Despite these low concentrations, proteins have a great technological relevance in winemaking as some of them, the grape pathogenesis-related (PR) proteins, can aggregate to form a visible haze. Among the grape PR-proteins, the thaumatin-like proteins (TLPs) and chitinases can undergo changes in structural integrity, particularly under certain conditions such as when wines are exposed to elevated temperatures during storage or transportation. In this paper the crystal structure and some physico-chemical parameters relevant for the haze formation mechanism of three isoforms of TLPs isolated from grape juice were determined. Plant TLPs generally have three domains and a cleft located between domains I and II.

Domain I is the largest and is made of 11 β-strands (β2, β3, β5, β8, β9, and β14 on the front; β1, β4, β10, β11, and β14 on the back), forming a β-sandwich of two β-sheets. The two β-sheets are stabilized by four disulfide bonds (residues 33–221, 89–95, 136–210, and 141–193). Domain II consists of a long α-helix (α4) and four α-helical segments (α1, α2, α3, and α5), and is stabilized by four disulfide bonds (residues 141–193, 149–159, 163–172, 173–180). The short domain III comprised 33 amino acid residues (residues 72–105), and includes a long loop and 2 β-strands (β6 and β7). This domain is stabilized by two disulfide bonds (residues 74–84, 89–95). Two disulfide bonds are shared by different domains: disulfide bond 89–95 connects domain I to III, while bond 141–193 connects domain I to II. Isoform differences in heat stability have practical and economic ramifications for winemaking. However, from the structures of the three proteins, it is clear that they only significantly differ in two loop regions. From the detailed analysis of their structural features it appears that the difference in function among proteins is attributable to the differences observed in a loop located between β-strands 9 and 10 and of the neighbouring regions.

> ATFNIQNHCSYTVWAAAVPGGGMQLGSGQSWSLNVNAGTTGGRVWARTNCNFDASGNGKCETGDCGGLLQCTAYGTPPNTLAEFALNQFSNLDFFDISLVDGFNVPMAFNPTSNGCTRGISCTADIVGECPAALKTTGGCNNPCTVFKTDEYCCNSGSCSATDYSRFFKTRCPDAYSYPKDDQTSTFTCTAGTNYEVVFCP>XSLTHRKFGGSGGSPFSGLSSIAVRSGSYLDAIIIDGVHHGGSGGNLSPTFTFGSGEYISNMTIRSGDYIDNISFETNMGRRFGPYGGSGGSANTLSNVKVIQINGSAGDYL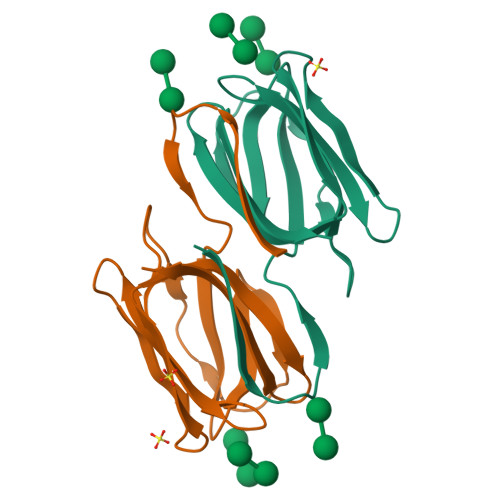DSLDIYYEQY[2x]> TL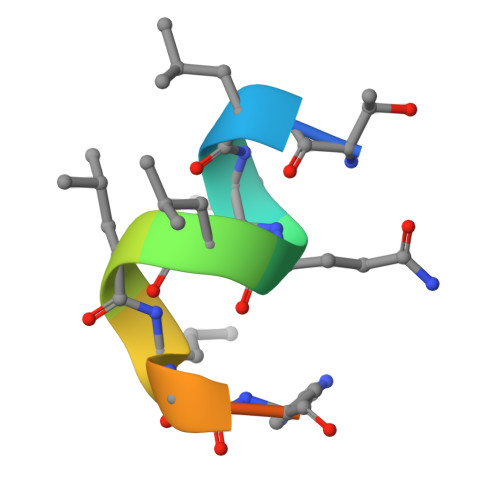LQLLLGHKNE>[8x]GMLTYQVKQGDTLNSIAADFRISTAALLQANPSLQAGLTAGQSIVIPGLPDPYTIPYHIAVSIGAKTLTLSL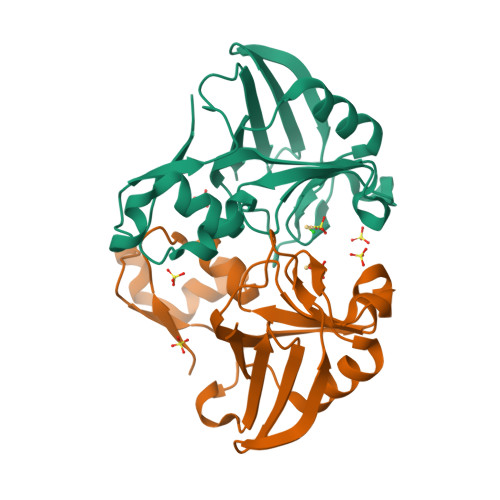NNRVMKTYPIAVGKILTQTPTGEFYIINRQRNPGGPFGAYWLSLSAAHYGIHGTNNPASIGKAVSKGCIRMHNKDVIELASIVPNGTRVTINR> MLAKKLALARSQGKPDPFKKDEFPLLQHIAVEVVSQNYILYPDLKGVPENVRDTIISKITTDLDILTMAPNIDQESFWQRACKNRWEKSQKSINIEEHGRSWKVAYLERYMEEFLTNIQNADDPNKKQILQAELKAAASWIHTLNLQNINQNIDIDFICKYLPLLTSLTLTYGTKYSGMDYNKQSVGMKLSEAANLGEAIKNCYSLLSLNISANMIDDDLLRFIMAGVNMNISLIELNLSHNKIEDQGARRIAKFLMRNEILLYLNLGNNLIGYEGSRYLAQALKVNKNLQSLNLKLNNLGDKAGKKLFQDLMLNKTLLELDVSGNQFEFETALKLSDYVADSMCGLKVLNIANNDFNDSCYENLKTGFTKNYSLAKLDLRGNKFSKTQEEKEQELKDPFRMFNLSQTEKELTQ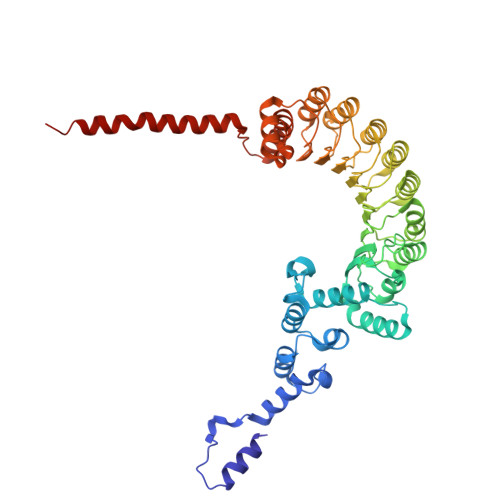IIIRHDLTAQKIQFFSESDLDKIKQLKELQGAKQEPEKVIQQDQNKE>[2x]GMVFQHDIYAGQQVLVTGGSSGIGAAIAMQFAELGAEVVALGLDADGVHAPRHPRIRREELDITDSQRLQRLFEALPRLDVLVNNAGISRDREEYDLATFERVLRLNLSA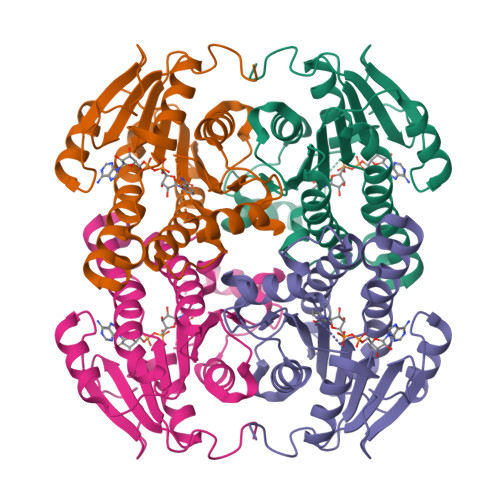AMLASQLARPLLAQRGGSILNIASMYSTFGSADRPAYSASKGAIVQLTRSLACEYAAERIRVNAIAPGWIDTPLGAGLKADVEATRRIMQRTPLARWGEAPEVASAAAFLCGPGASFVTGAVLAVDGGYLCA> SPQREPQRVSHEQFRAALQLVVDPGDPRSYLDNFIKIGEGSTGIVCIATVRSSGKLVAVKKMDLRKQQRREL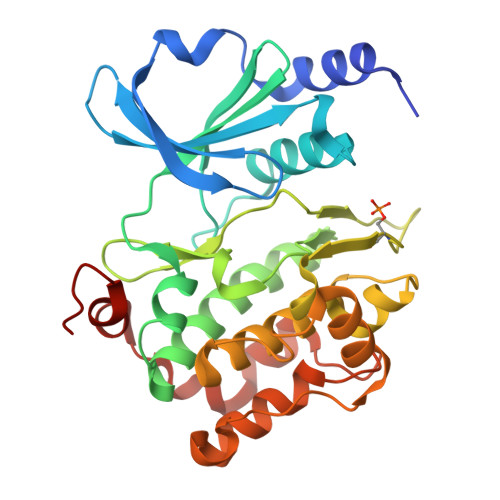LFNEVVIMRDYQHENVVEMYNSYLVGDELWVVMEFLEGGALTDIVTHTRMNEEQIAAVCLAVLQALSVLHAQGVIHRDIKSDSILLTHDGRVKLSDFGFCAQVSKEVPRRKSLVGTPYWMAPELISRLPYGPEVDIWSLGIMVIEMVDGEPPYFNEPPLKAMKMIRDNLPPRLKNLHKVSPSLKGFLDRLLVRDPAQRATAAELLKHPFLAKAGPPASIVPLMRQNRTR>GPLGSPEFMALDDDIRILGTVGLFESFTPEQLRLLAFGAERLVLRAGRELFREGQSADCAYIIVTGTITLFHEGDEGRVTIRPVGPGAILGEM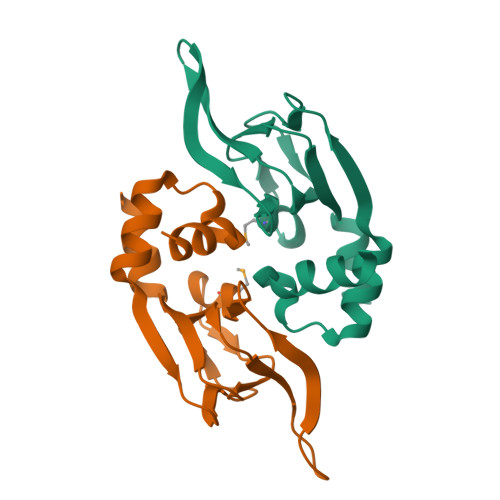ALIAQTTRLTGAVADVETEVIRISRSIFRRILEEYPEV[2x]The non-LEE encoded effector protein B (NleB) has GT activity and inhibits NF-κB activation by transferring N-acetyl glucosamine (GlcNAc) to host death domain-containing proteins and to glyceraldehyde 3-phosphate dehydrogenase (GAPDH). The glycosylation target is an arginine residue, which was unexpected because the guanidine group of arginine is nucleophilically poor at physiological pH. The T3SS effectors SseK1 and SseK2 from Salmonella typhimurium SL1344 are NleB orthologs that behave as NleB1-like GTs, although they differ in protein substrate specificity. Here, by using a combination of X-ray crystallography, STD-NMR, enzyme kinetics, molecular dynamics simulations, and in vivo experiments, we show that these enzymes are GT-A fold retaining GTs that most likely follow an SNi mechanism.

SseK2 was solved both in its unliganded form and in complex with UDP and UDP-GlcNAc. Therefore, the electron density map for this domain was not resolved. However, in the structures with UDP and UDP-GlcNAc, the substrate leads to an unambiguous electron density map for the C-terminal lid domain, implying that the domain is well ordered only in the presence of the nucleotide (detailed information is described below). To obtain insight into the importance of these residues in substrate recognition, we conducted in-silico docking of the acceptor Arg to the SseK2-UDP crystal structure. It was observed that a closed conformation of SseK2 structure possesses a putative acceptor substrate binding site pocket that is connected to the anomeric carbon of GlcNAc. As a result, the negatively charged pocket of the concave active site interacts with the positively charged guanidine group. In particular, Glu271, the β-phosphate of UDP, and His260 were located in a position suitable for hydrogen bonding. In the docking structure of SseK2, a single negatively charged residue (Glu271SseK2) and an additional β-phosphate from UDP are in close contact to the guanidinium group of the acceptor Arg. In addition, His260SseK2 is located near the guanidinium group of the acceptor Arg.

>[2x]MARFNAAFTRIKIMFSRIRGLISCQSNTQTIAPTLSPPSSGHVSFAGIDYPLLPLNHQTPLVFQWFERNPDRFGQNEIPIINTQKNPYLNNIINAAIIEKERIIGIFVDGDFSKGQRKALGKLEQNYRNIKVIYNSDLNYSMYDKKLTTIYLENITKLEAQSASERDEVLLNGVKKSLEDVLKNNPEETLISSHNKDKGHLWFDFYRNLFLLKGSDAFLEAGKPGCHHLQPGGGCIYLDADMLLTDKLGTLYLPDGIAIHVSRKDNHVSLENGIIAVNRSEHPALIKGLEIMHSKPYGDPYNDWLSKGLRHYFDGSHIQDYDAFCDFIEFKHENIIMNTSSLTASSWR>MENQLTKSVEERTFQYQDSLPSLPVPALEESLKKYLESVKPFANEDEYKKTEEIVQKFQEGAGKRLHQKLLERARGKRNWLEEWWLNVAYLDVRIPSQLNVNFVGPCPHFEHYWPAREGTQLERGSMMLWHNLNYWQLLRREKLPVHKSGNTPLDMNQFRMLFSTCKVPGITRDSIMNYFKTESEGHCPTHIAVLCRGRAFVFDVLHEGCLITPPELLRQLTYIHKKCSNEPVGPSIAALTSEERTRW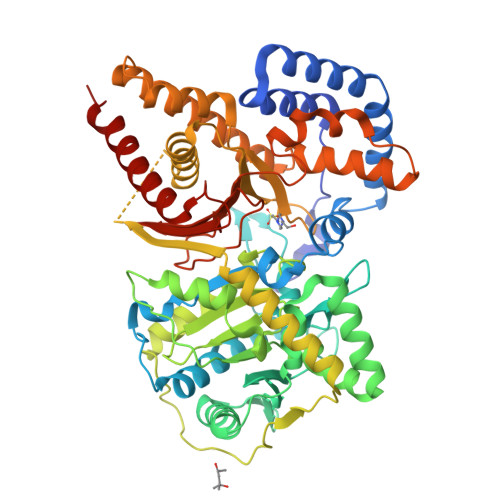AKAREYLISLDPENLTLLEKIQTSLFVYSIEDSSPHATPEEYSQVFEMLLGGDPSVRWGDKSYNLISFANGIFGCCCDHAPYDAMVVVNIAHYVDERVLETEGRWKGSEKVRDIPLPEELVFTVDEKILNDVSQAKAQHLKAASDLQIAASTFTSFGKKLTKEEALHPDTFIQLALQLAYYRLHGRPGCCYETAMTRYFYHGRTETVRSCTVEAVRWCQSMQDPSASLLERQQKMLEAFAKHNKMMKDCSHGKGFDRHLLGLLLIAKEEGLPVPELFEDPLFSRSGGGGNFVLSTSLVGYLRVQGVVVPMVHNGYGFFYHIRDDRFVVACSSWRSCPETDAEKLVQMIFHAFHDMIQLMNTAHL[2x]>[8x]PLREAKDLHTALHIGPRALSKACNISMQQAREVVQTCPHCNSAPALEAGVNPRGLGPLQIWQTDFTLEPRMAPRSWLAVTVDTASSAIVVTQHGRVTSVAVQHHWATAIAVLGRPKAIKTDNGSCFTSKSTREWLARWGIAHTTGIPGNSQGQAMVERANRLLKDKIRVLAEGDGFMKRIPTSKQGELLAKAMYALNHFERGENTKTPIQKHWRPTVLTEGPPVKIRIETGEWEKGWNVLVWGR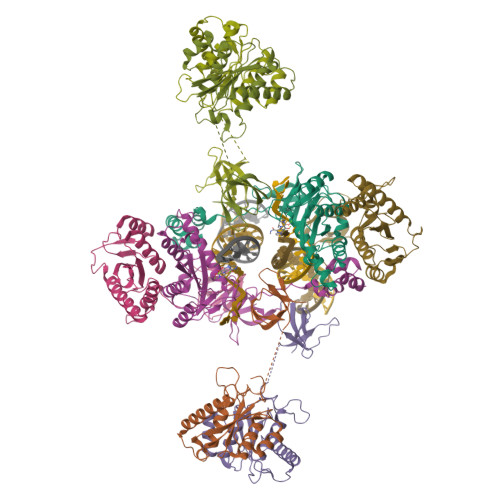GYAAVKNRDTDKVIWVPSRKVKPDITQKDEVTKK>[6x]MSLKWFNTLSHNRWLEQETDRIFNFGKNAVVPTGFGWLGNKGQIKEEMGTHLWITARMLHVYSVAASMGRPGAYDLVDHGIKAMNGALRDKKYGGWYA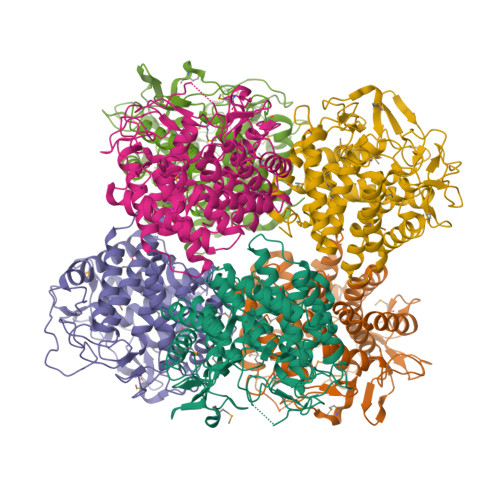CVNDQGVVDASKQGYQHFFALLGAASAVTTGHPEARKLLDYTIEVIEKYFWSEEEQMCLESWDEAFSQTEDYRGGNANMHAVEAFLIVYDVTHDKKWLDRALRIASVIIHDVARNGDYRVNEHFDSQWNPIRDYNKDNPAHRFRAYGGTPGHWIEWGRLMLHLHAALEARFETPPAWLLEDAKGLFHATIRDAWAPDGADGFVYSVDWDGKPIVRERVRWPIVEAMGTAYALYTLTDDSQYEEWYQKWWDYCIKYLMDYENGSWWQELDADNKVTTKVWDGKQDIYHLLHCLVIPRLPLAPGLAPAVAAGLLDINAKEGGSHHHHHH Amaryllidaceae alkaloids, such as the Alzheimer’s medication galantamine, are complex plant secondary metabolites with recognized therapeutic value. 4′-O-methylnorbelladine (4NB) is the branchpoint intermediate for the entire amaryllidaceae alkaloid (AA) family, and therefore was the target compound for biosensor generation. Since norbelladine 4′-O-methyltransferase (Nb4OMT) from the wild daffodil Narcissus sp. aff. pseudonarcissus, is directly responsible for 4NB production from norbelladine, we chose this as a starting point for development of a fuller pathway. Furthermore, LC/MS analysis identified 3’-O-Methylnorbelladine as a minor component, indicating that the wild-type Nb4OMT enzyme was not highly regiospecific.

To better understand the mechanism underlying the three beneficial substitutions in the Nb4OMTE36P/G40E/A53M variant, we determined the structure of the Nb4OMTE36P/G40E/A53M variant in complex with S-adenosyl-L-homocysteine (SAH) at 2.4 Å resolution. The Nb4OMT variant exists as a homodimer in the crystalline form, consistent with its size exclusion chromatogram. The overall fold of the protein was almost identical to the predicted AlphaFold2 structure, except for the N-terminal region. AlphaFold2 predicts that Lys13 forms tight salt bridge interaction with Asp155, Asp181, and Asn182 in the enzyme active site, while the experimental structure showed that Asp155, Asp181, and Asn182 instead coordinate a Ca2+ ion and Lys13 forms hydrogen bonds with the backbone of Tyr186 and the sidechain of Tyr194. The experimental structure of Nb4OMTE36P/G40E/A53M provides a basis for the improved thermostability of the enzyme (an increase in Tm from 52.8 °C to 58.4 °C). The A53M substitution inserts a larger hydrophobic methionine inside the hydrophobic pocket formed by Trp50, Tyr81, and Tyr108, stabilizing the active site of Nb4OMT. The E36P-G40E double mutant shifts a glutamate from position 36 to position 40 and thereby preserves the salt bridge interaction with Lys118 while proline capping the alpha helix. To better determine how the A53M substitution affects the substrate recognition of Nb4OMT, GNINA 1.0 was used to dock norbelladine into the crystal structure of Nb4OMTE36P/G40E/A53M with SAH and Ca2+ already in the active site (based on Fo-Fc electron densities). In the docked structure, the Ca2+ ion positions the catechol moiety of the substrate adjacent to the SAH binding site. A sulfur-π interaction between the catechol group of norbelladine and Methionine 53 may also restrict the rotation of the catechol group, thereby reducing the cross-methylation of the 3’ position and improving specificity.

>[6x]MGASIDDYSLVHKNILHSEDLLKYILETSAYPREHPQLKELREVTEKHEWSSMLVPADEGLFLSMLLKLMNAKRTIEIGVYTGYSLLTTALALPEDGKITAIDVNKSYYEIGLPFIQKAGVEHKINFIESEALPVLDQMLEEMKEEDLYDYAFVDADKSNYANYHERLVKLVRIGGAILYDNTLWYGSVAYPEYPGLHPEEEVARLSFRNLNTFLAADPRVEISQVSIGDGVTICRRLY> MSQVKRANENRETARFIKKHKKQVTNPIDEKNGTSNCIVRVPIALYVSLAPMYLENPLQGVMKQHLNPLVMKYNNKVGGVVLGYEGLKILDADPLSKEDTSEKLIKITPDTPFGFTWCHVNLYVWQPQVGDVLEGYIFIQSASHIGLLIHDAFNASIKKNNIPVDWTFVHNDGNRSLGHW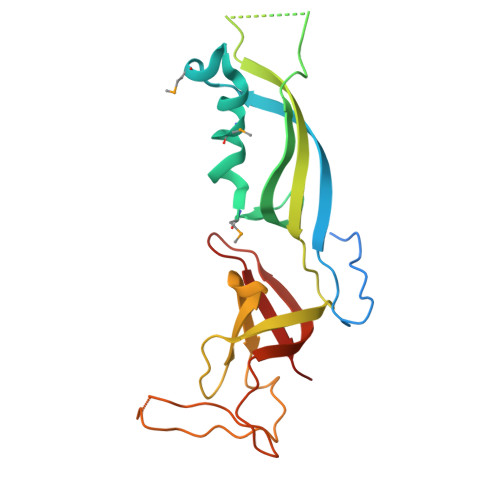VDSNGEPIDGKLRFTVRNVHTTGRVVSVDGTLIS> MNQHLLGNPKLTVTHVNEVKAGINHIVVDSVQYGNQEMIMEKDGTVEMRDGEKLYINIFRPNKDGKFPVVMSADTYGKDNKPKITNMGALWPTLGTIPTSSFTPEESPDPGFWVPNDYVVVKVALRGSDKSKGVLSPWSKREAEDYYEVIEWAANQSWSNGNIGTNGVSYLAVTQWWVASLNPPHLKAMIPWEGLNDMYREVAFHGGIPDTGFYRFWTQGIFARWTDNPNIEDLIQAQQEHPLFDDFWKQRQVPLSQIKTPLLTCASWSTQGLHNRGSFEGFKQAASEEKWLYVHGRKEWESYYARENLERQKSFFDFYLKEENNDWKDTPHVIYEVRDQFYKGEFKSASAFPLPNAEYTPLYLNAENHTLNHAKISSAHVAQYDSEDKQQDVSFKYTFDKDTELVGNMNLKLWVSTKDSDDMDLFAGIKKLDRRGNEVNFPDFNHIENGQVATGWLRVSHRELDQEKSSIAQPWHKHETELKLSQDEIVPVEIEL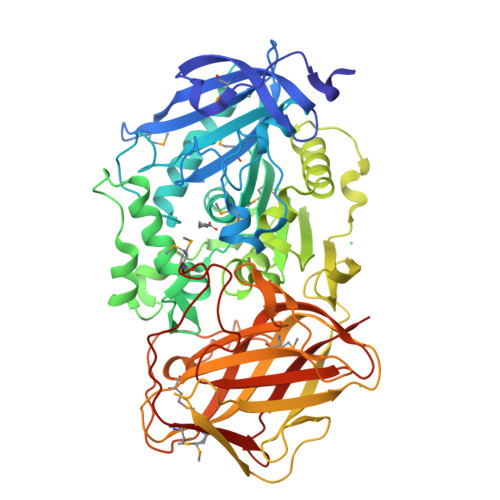LPSGTLFKQGETLEVVVKGSEIVIGNSTPGMKTRYEHEETVNKGMHMIYTGGKYDSQLIIPIVN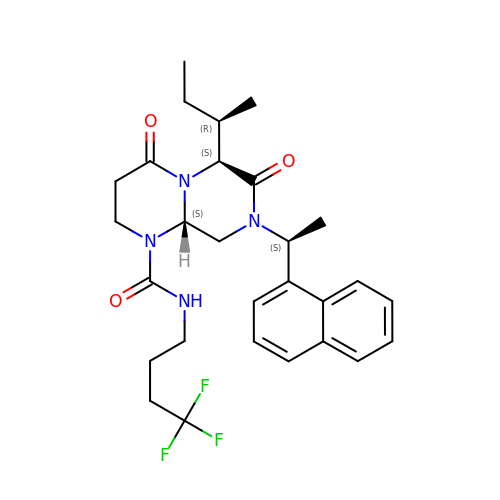(6S,9aS)-6-[(2R)-butan-2-yl]-8-[(1S)-1-naphthalen-1-ylethyl]-4,7-bis(oxidanylidene)-N-[4,4,4-tris(fluoranyl)butyl]-3,6,9,9a-tetrahydro-2H-pyrazino[1,2-a]pyrimidine-1-carboxamide | C28 H35 F3 N4 O3 | BAZGDIOJCKGDHH-UXELZNRMSA-N> GNVLEFATLDSKRNVNDTEVESMDSQAYKKELIEQIMIAQTECSLALDMTSLLLSKFKENSIETISPFLKSTVPPSSLQFSRSQPPESKESDATLAKCWKEKSLTSSCKFLFEAKERLTSVVETEHEYYTELVKVKEASWPLFNSQGSNHLSVQYSCLGGISLGLGLIRMKPESKSFEVQSSLLYSQAALKISILNKDRDEIGSSTWSWPSQNCNSVLLKDIYKLQEILFEMDIWNSLLQEAQSCGNQGVNFTGDEILVPISDDHVVRITLETSSKNTESGFTEDKKSNEDTSTNFVTIKQEKELLKCLCDTLNAIAHILFLKHCRKSDRRSQQPELYMAIDANAPLILRPLIFYYNLNQESLEFQRWLKQRDISFKFMPNYPWEKAKDFLELENSLSINRLS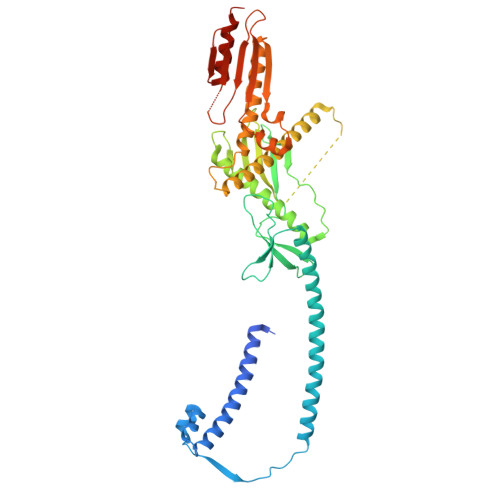ISWRIMVSNFEPAIFIQHTPTLHGTDKSVWRCKDQYSSNQFSSLKNVCQYIEHHINSLSRRSKKTE> MGYFELQLSALRNVNGELLSGACCDGDGRTTRAGGCGHDECDTYVRVCLKEYQAKVTPTGPCSYGHGATPVLGGNSFYLPPAGAAGDRARARARAGGDQDPGLVVIPFQFAWPRSFTLIVEAWDWDNDTTPNEELLIERVSHAGMINPEDRWKSLHFSGHVAHLELQIRVR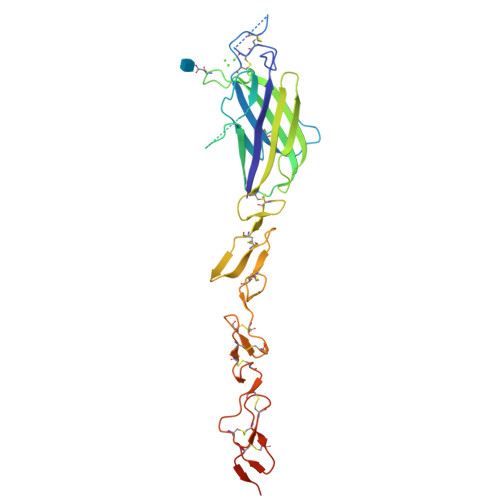CDENYYSATCNKFCRPRNDFFGHYTCDQYGNKACMDGWMGKECKEAVCKQGCNLLHGGCTVPGECRCSYGWQGRFCDECVPYPGCVHGSCVEPWQCNCETNWGGLLCDKDLNGSHHHHHHHH> MDKKDDVKETIKKSKTIDATKYEMWTYVNLETGQTETHRDFSEWH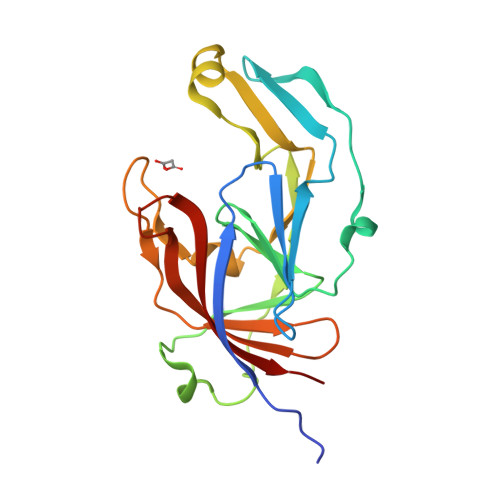VMKNGKLLETIPAKGSEADIKIKWHIAIHRFDIRTNEGEAIATKETEFSKVTGLPAGDYKKDVEIKDKMLVGFNMADMMKSKFTVAGMAKVNPVLKTWIVENPMGKAPVLSKSVFVVKFKDGSYAKIKFTDATNDKQEKGHVSFNYEFQPK Here, we report the atomic structures of an engineered diffocin, a contractile syringe-like molecular machine that kills the Gram-positive bacterium Clostridioides difficile. Captured in one pre-contraction and two post-contraction states, each structure fashions six proteins in the bacteria-targeting baseplate, two proteins in the energy-storing trunk, and a collar linking the sheath with the membrane-penetrating tube. Specific attachment of baseplate tail fibers to receptors on the surface of a target bacterial cell triggers conformational changes of the neighboring baseplate, which leads to reorientation of sheath proteins and contraction of the entire sheath assembly. Since the sheath and the tube are anchored together at the opposite end by the collar, collapsing the sheath pushes the tube through the baseplate, driving it to puncture the cell wall and underlying cytoplasmic membrane.

There is a symmetry mismatch among the three major parts of the diffocin: the collar (C6 symmetry), the trunk (C6+helical symmetry), and the baseplate (C6 + C3 symmetry). By applying the corresponding symmetry during single-particle reconstructions, we determined cryoEM structures of the collar, trunk, and baseplate regions of pre-contraction diffocin separately at resolutions of 2.7 Å, 2.2 Å, and 2.6 Å, respectively. The inner tube and outer sheath are tethered together by a hexameric ring of collar protein (CD1362) at the collar-proximal end of the diffocin. The N-terminal domain of the collar subunit binds to the tube, while its C-terminal β-strand extends towards the C-terminal β-hairpin of last sheath, forming a three-β-strand handshake interaction. These interfaces are maintained during contraction, enabling the collar to function as a force transducer between sheath contraction and tube ejection. We define these conformations as conformers A, B, C, and D. As the trunk assembles from the baseplate to the collar, conformer A forms the first layer, followed by alternating contributions from conformers B and C, and finally, conformer D terminates the sheath by interacting with the collar. The density of the TMP ends at the collar region and it displays higher flexibility. In summary, the diffocin TMP assembles as a trimer with a coiled-coil pattern, with the N-termini interacting with the collar and the C-termini anchored on the spike.

>MAIGLPSINISFKELATTVKERSARGIIAMVLKDAKALGLNEIHEKEDIPVDLSAENKEYINLALMGNVNTPNKLLVYVIEGEADIQTALDFLETKEFNYLCMPKAVEADKTAIKNWIIKLRDIDKVKVKAVLGKVVGNHEGIINFTTEDVLVGEKKYSVDEFTSRVAGLIAGTPLSQSVTYTKLSDVVDIPKMTKVDAESRVNKGELILIKEAGAIRIARGVNSLTELTAEKGEMFQKIKIVDTLDIIHSDIRKVIIDDYIGKVTNSYDNKCLLIVAIKSYLEELEKSALIESDSTVEIDFEAQKSYLKSKGVDLSYMTLQEIKEANTGSKVFLKAKIKVLDAMEDIDLSIEI[18x];>MANMEARNVMSGTWGELWLDGNKVAEVKKFQAKMEFTKEDIIIAGQMGTDTKYMGYKGKGSITLYHVSSRMHKLIGEKIKRGSEPRFVAISKLNDPDSYGAERIAVKNIAFDDLTLADWEVGVKGEIEAPFTFTEYDFLDII[18x];>[6x]MLKYKEILETIIEILKKNFTESIFIDDESVQGSEGSCFFVSILSVICTPVMLNTNNKDIVISIKYLPKPQSKSIRMYEISDELNKLFNRNIKVTDRKLNITKLEQSIKKEESIYVLNFTFTLNYLDSVYEEDVVYENMKEINLNLGE> MSKIFVNPSAIRAGLADLEMAEETVDLINRNIEDNQAHLQGEPIEVDSLPEDENLYFQGMDADRIVFRSNNQVVSLRPEIIADQYEYKYPAIKDLKKPCITLGKAPDLNKAYKSVLSGMNAAKLDPDDVCSYLAAAMQFFEGTCPEDWTSYGILIARKGDKITPNSLVEIKRNDVEGNWALTGGMEMTRDPTVSE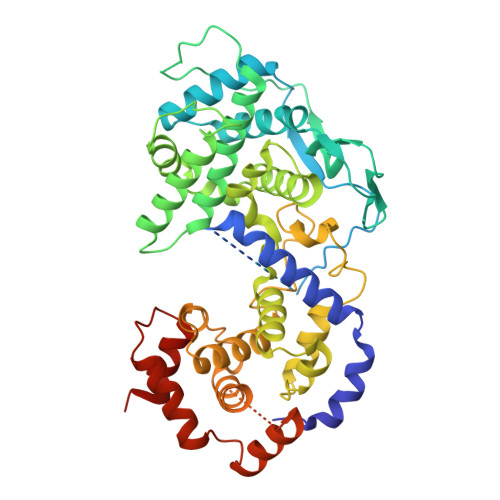HASLVGLLLSLYRLSKISGQNTGNYKTNIADRIEQIFETAPFVKIVEHHTLMTTHKMCANWSTIPNFRFLAGTYDMFFSRIEHLYSAIRVGTVVTAYEDCSGLVSFTGFIKQINLTAREAILYFFHKNFEEEIRRMLEPGQETAVPHSYFIHFRSLGLSGKSPYSSNAVGHVFNLIHFVGCYMGQIRSLNATVIAACAPHEMSVLGGYLGEEFFGRGTFERRFFRDEKELQEYEAAELTKTDVALADDGTVDSDDEDHLSGEARGPEAVYARIMMNGGRLKRSHIRRYVSVSSNHQARPNSFAEFLNKTYSSDSHHHHHHHH Phylogenetically diverse bacteria can carry out chloramphenicol reduction, but only a single enzyme has been described that efficiently catalyzes this reaction, the NfsB nitroreductase from Haemophilus influenzae strain KW20. We found that expression of H. influenzae and Neisseria spp. nfsB genes, but not Pasteurella multocida nfsB, allows Escherichia coli to resist chloramphenicol by nitroreduction. Mass spectrometric analysis confirmed that purified H. influenzae and N. meningitides NfsB enzymes reduce chloramphenicol to amino-chloramphenicol, while kinetics analyses supported the hypothesis that chloramphenicol reduction is a secondary activity. Previous kinetic studies of nitroreductase catalysis revealed that reactions progress by a double-displacement (ping-pong) mechanism that appears to lack the gating steps necessary to impose specificity, explaining the substrate promiscuity of these enzymes.

To understand better how variation in the substrate-binding site mediates activity, we solved the crystal structures of the NfsB homologs from Hi KW20, Hi Int1, Hi 86-028NP, and Nm Z2491. The Hi Int1 and Hi 86-028NP enzymes showed comparable, although statistically significant, kinetics (q < 0.05) to Hi KW20 NfsB. The relative increase in resistance conferred by H. influenzae or Neisseria nfsB expression ranged from approximately a 16-fold increase (Hi KW20 and Hi 86-028NP) down to an ∼2-fold increase (Hi Int1 and Hi 12). The divergence in chloramphenicol resistance and in vitro activity likely reflect the vagaries of heterologous expression in Es. coli and suggest the presence of important subtleties that still need to be accounted for when estimating mobilization risks of cryptic and proto-resistance genes. This is especially evident with the NfsB enzymes from Hi KW20 and Hi Int1. A molecular explanation for this difference remains to be determined. Intuitively, the Ser68-Met74 pair found in Hi 12 NfsB would provide more of the flexibility needed to properly locate and orient Trp71 to make space for the ribose of NADP than the Pro68-Ile74 pair in other H. influenzae NfsB homologs (Pro68-Ala74 in Nm Z2491 NfsB).

>[2x]SNAMTQLTREQVLELFHQRSSTRYYDPTKKISDEDFECILECGRLSPSSVGSEPWKFLVIQNKTLREKMKPFSWGMINQLDNCSHLVVILAKKNARYDSPFFVDVMARKGLNAEQQQAALAKYKALQEEDMKLLENDRTLFDWCSKQTYIALANMLTGASALGIDSCPIEGFHYDKMNECLAEEGLFDPQEYAVSVAATFGYRSRDIAKKSRKTLDEVVKWVG>RCLF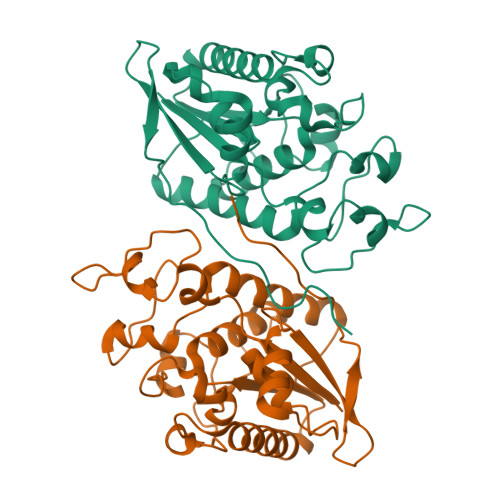VCRHGERMDVVFGKYWLSQCFDAKGRYIRTNLNMPHSLPQRSGGFRDYEKDAPITVFGCMQARLVGEALLESNTVIDHVYCSPSLRCVQTAHNILKGLQQDNHLKIRVEPGLFEWTKWVAGSTLPAWIPPSELAAANLSVDTTYRPHIPVSKLAISESYDTYINRSFQVTKEIISECKSKGNNILIVAHASSLEACTCQLQGLSPQNSKDFVQMVRKIPYLGFCSCEELGETGIWQLTDPPILPLTHGPTGGFNWRE[3x]>MSDSTPKTPRGFVVHTAPVGLADDGRDDFTVLASTAPATVSAVFTRSRFAGPSVVLCREAVADGQARGVVVLARNANVATGLEGEENAREVREAVARALGLPEGEMLIASTGVIGRQYPMESIREHLKTLEWPAGEGGFDRAARAIMTTDTRPKEVRVSVGGATL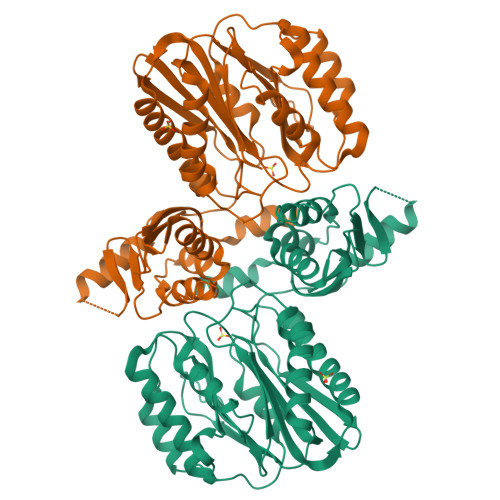VGIAKGVGMLEPDMATLLTFFATDARLDPAEQDRLFRRVMDRTFNAVSIDTDTSTSDTAVLFANGLAGEVDAGEFEEALHTAALALVKDIASDGEGAAKLIEVQVTGARDDAQAKRVGKTVVNSPLVKTAVHGCDPNWGRVAMAIGKCSDDTDIDQERVTIRFGEVEVYPPKARGDQADDALRAAVAEHLRGDEVVIGIDLAIADGAFTVYGCDLTEGYVRLNSEYTT[2x]The intrinsic pathway to apoptosis is regulated by interactions between members of three factions of the Bcl-2 protein family: the BH3-only proteins such as Bim and Bid, which initiate the process, the essential effectors Bax and Bak, and the prosurvival members, which oppose the action of both other factions. Unlike Bak, which is constitutively anchored in the mitochondrial outer membrane (MOM) via its C-terminal segment, Bax is largely cytosolic in healthy cells and accumulates at the MOM only upon a death signal. Core/latch dimers of Bax and Bak form on treatment of the monomeric proteins with certain BH3 peptides and CHAPS, and Bax and Bak core domains form symmetric homodimers, supporting that unlatching the core domain is a necessary step to Bax and Bak oligomerisation and permeabilisation of the MOM. Bim and Bid are both potent direct activators of Bax, but Bim is less dependent on interactions via its ‘h0' residues than is Bid.

We previously showed that mini-BH3 motifs, 20-mers spanning residues ‘h0'–‘h4', sufficed to trigger dissociation of BaxΔC into core and latch domains. To confirm that the N- and C-terminal segments of the longer peptides did not influence the peptides' interaction with Bax, we crystallised both BimBH3mini and BidBH3mini with BaxΔC26. These structures are essentially identical to that reported above and to BidBH3:BaxΔC21 (PDB 4BD27), except to note that in the case of the BimBH3mini complex, no clear density is evident for F159 (the ‘h4' residue). The BH3mini:BaxΔC26 complexes contain a cavity between helices α1, α2, α5 and α8 (shaped with the side chains of residues 26, 30, 60, 63, 66, 67, 110, 111, 114, 115, 158 and 161) as observed also in the BidBH3:BaxΔC21 complex but not in the apo BaxΔC21 core/latch dimer.

> MDGSGEQPRGGGPTSSEQIMKTGALLLQGFIQDRAGRMGGEAPELALDPVPQDASTKKLSESLKRIGDELDSNMELQRMIAAVDTDSPREVFFRVAADMFSDGNFNWGRVVALFYFASKLVLKALSTKVPELIRTIMGWTLDFLRERLLGWIQDQGGWDGLLSYFGSS;> XQEDIIRNIARHLAQVGDSMD The γ-tubulin ring complex (γ-TuRC) acts as a structural template for microtubule formation at centrosomes, associating with two main compartments: the pericentriolar material and the centriole lumen. The γ-TuRC has a helical shape consisting of 14 spokes, each containing a copy of γ-tubulin presented by the C-terminal gamma ring protein 2 (GRIP2) domain of one of five paralogous γ-tubulin complex proteins (GCPs). The GCP proteins interact via their N-terminal GRIP1 domains in a specific order: the γ-TuRC core harbors four pairs of GCP2/GCP3 (spoke 1–8), followed by a sequence of vertebrate-specific paralogs GCP4/GCP5/GCP4/GCP6 (spoke 9-12) and finally another pair of GCP2/GCP3 (spoke 13-14). The inside of the γ-TuRC is lined by a lumenal bridge composed of one actin molecule, as well as two α-helical modules formed by the microprotein MZT1 (mitotic-spindle organizing protein 1) and the N-terminal extensions of GCP3 and GCP6 (N-GCP3 and N-GCP6), respectively.

We subjected the purified X. laevis γ-TuRCs to cryo-EM SPA and identified a subset of particles with stoichiometric NEDD1/N-GCP3/MZT1 grapnel density. We, therefore, subjected the NEDD1/N-GCP3/MZT1 density segment to focused refinement (see “Methods”), improving local resolution for NEDD1 to 4-5 Å. The very C-terminal NEDD1 helix segments were an exception, as they were predicted straight, but are kinked in the cryo-EM reconstruction. After optimizing the model by another round of MDFF into the density obtained by focused refinement, resolved bulky hydrophobic side chains and the length of resolved alpha-helices confirmed the density segment as NEDD1. Our cryo-EM reconstruction resolves a tetramer of the NEDD1 C-terminus, comprising two consecutive helices in each protomer (NEDD1598-648 and NEDD1651-670; all residue numbers refer to X. laevis proteins). At its center, NEDD1598-648 forms a tetrameric coiled-coil that provides the binding site for four N-GCP3/MZT1 modules. The interaction between NEDD1 and the N-GCP3/MZT1 modules is characterized by complementary charged and hydrophobic patches. In addition to direct interaction with NEDD1, the N-GCP3/MZT1 modules also share an extensive interaction surface with each other, suggesting cooperative binding of N-GCP3/MZT1 modules to NEDD1. In contrast to NEDD1598-648, the NEDD1651-670 helix breaks the fourfold symmetry and forms two small dimeric coiled-coils that splay out from each other. One protomer in the upper dimer of NEDD1651-670 contacts GCP6223-240, which is part of a larger region of N-GCP6 that lines the inside of GRIP1 domains of spoke 1 and 2. The lower dimer of NEDD1651-670 appears to make little to no contact to spoke 1 and 2, but its conformation is likely stabilized by an unidentified wedge density between the upper and lower NEDD1651-670 dimers.

>MSEFRIHHDVNELISLLHVFGLEGADVYIDLLQKNRTPYVTTSVSTHSAKVKIAEFSRTPDDFLKKYEELKSKNTRNLDPLVYLLSKLIEDKETLQYLQQNAKDKAELATSSVTSVSLPIAPNTSKISMQELEELRRQLETATVAVSCSHQPVEVLRKFLRDKLNKKHTGHPVPVFPSWVYERPALTGDFMSFSNPSTDVTVSIGTLPLPSQETCLVEDLLYILIGVDGRYISVQPLVGRQSRSFSVEQNLDSSVKELVNRILPVATNYSTVTRFVEENSSFEYGQVNHALGAAMRTLGKEYMILISQLEHLQRQGLLSLQKLWFYIQPTLRTMEVLASIATSLNKGECFGGATLSLLHDRTFGYTGDSQAQELCLYLTKAASAPYFDILERWIYRGIINDPYSEFMVEEHELQKEKIQEDYNDKYWDQRYTIVQQQIPSFLQKVADKILSTGKYLNVVRECGHDVTCPDAKEITYTLKEQAYVERIEKAYNYASKVLLDFLMEEEELVAHLRSIKHYFLMDQGDFFVHFMDLTEEELKKPVDDIIPTRLEALLELALRMSTANTDPFKDDLKIELMPHDLITQLLRVLAIETHQEKALINSDPTELALSGLESFSFDYIVKWPLSLIINRKALTRYQMLFRHMFYCKHVERLLCNVWISNKTAKQFSLHSAKWFAGAFTLRQRMLNFVQNIQYYMMFEVMEPTWHILEKNLKSASNIDDVLSHHTSFLDNCLKDCMLTNPELLKIFSKLMSVCVMFTNCLQRFTQSMQVQTEMEHLTLEHGTMMGPPTQCERTEEALKKKLTSKYLEEHIDKFPSSFGFESTINNFDSNFSAHLMDLLDKLSMYSTSDCEHSMINIIYRLDFNGFYTERLKQLSSERNQKSAPLLGPAQHAVSTK[4x];>[9x]MAVPDQKSPNVLLQNLCCRILGKGEADVAQQFQYAVRVIGSNFAPTVERDEFLVTEKIKKEFVRQRREADGALFSELHRKLQSQGVLKNRWSILYLLLSLSEDPRKQPNKTSSFAALFAQALPRDAHSTPYYYARPQSLPLSYQDRNVQCAQNAASIGSSGISSIGMYALNGPTPQSIIQGQSNQTPNMGDALRQQLGSRLAWTLAAGQQPSQQSTTTKGLPNTVSRNVPRTRREGDSSGSVEITETSLVRDLLYVFQGIDGKFVKMCNSENCYKVDGKVAVSKSLKDITSKLSELGWLHNKIKKYTDQRSLDRAFGLVGQSFCAALHQELKEYYRLLSVLHSQLQVEDDQGVNLGVESSLTLRRLLVWTFDPKIRLKTLAALVDHCQGRKGGELASAVHAYTKTGDPYMRSLVQHILGLVAYPILNFLYRWIYDGELEDTYHEFFVASDPVVKTDRLWHDKYSLRKSMIPSFMTMDQSRKVLLIGKSINFLHQVCHDQTPASKAMAVGKSAESPKDAAELFTDLENAFQTKIDAAYFDTSKYLLDVLNKNYNLLEHMQAMRRYLLLGQGDFIRHLMDLLKPELVRPATTLYQHNLTGILETAVRATNAQFDNPEILKRLDVRLLEVSPGDTGWDVFSLDYHVDGPIATVFTRECMSHYLRVFNFLWRAKRMEYILTDIWKGHMCNAKLLKGMPELSGVLHQCHILASEMVHFIHQMQYYITFEVLECSWDELWNKVLKAQDLDHIIAAHDVFLDTIISRCLLDSESRALLNQLRAVFDQIIEFQNAQDALYRAALEELQQRLQFEERKKERESEGEWGVTAAEEDVENKRIQEFQESIPKMRSQLRILTHFYQGIVQQFLVLLTTSTDESLRFLSFRLDFNEHYKAREPRLRVSMGTRGRRSFHV;>MIHELLLALSGYPGSIFTWNKRTGLQVSQDIPFLHPGETSVLNRLCKLGTDYIRFTEFIEQYTGHVQQQDHHPSQQGQVGLHGIYLRAFCRGLDSILQPYRQALLDLEQEFLADPHLSISHINYSLDQFHLLFPSIMVVVEQIKSQKIHGCQILETVYKHSCGGLPPVRSALEKTLAVCHGVMYKQLSAWMLHGLLLDQYEEFFVRQGSSSGNLAAAFEEEEDDLGIGGLTGKQLRELQDLRLIEEENMLAPSLKQFSLRAEMLPSYIPVRVAEKILFVGESVQMFENQNVNMSRTGSILKNQEDTFAAELHRLKQQPLFSLVDFESVLDRIRSTVAEHLWKLMVEESDLLGQLKIIKDFYLLGRGELFQAFIDVAQNMLKTPPTAVTEHDVNVAFQLSAHKVLLDDDNLLPLLNLTIDYHGKEHKDTSQPREGPFRDMSPREAPTSGWAALGLSYKVQWPLHILFTPAVLEKYNVVFKYLLSVRRVQSELQHCWALQMQRKHLESNKTDAIKWRLQNHMAFLVDNLQYYLQVDVLESQFSQLLQQINSTRDFESIRLAHDHFLSNLLAQSFILLKPVFHCLNEILELCHSFCSLVSQNLGPLDERGAGQLDILVKGFSCQSSLLFRILSSVRNHQINPDLAQLLLRLDYNKYYTQAGGTLGSFGL[2x];> MAHWTRFERDQEGDIKKLVSLMSGIQDDQDGNFQQALQFAWSNFRFHRYLDVSSHTVLRTLEGIFEKLVVHSDLEKAESWKRLTEEFLLLPLPNTEGTKTDSHFAVLSLLLCLSDSPSNHDYTEKPRKKENDEQEPFDWGKYLREGEDIEFSPDADTPEWSEASEEEDAQEPPSREDSGIQVDRTPLEDPEKKGAPPLVSWKVGEPDARSWLEQHIVHQYWTSRAPRFSHSSHLHSNLSAIWDQHLYTTDPLYTPDDKTIVTETQVIRETLWLLSGVKKLLIFQLNDGKVNVRNDIIVTHMTQNCLRSVLEQIAAYGQVVFRLQKFIDEITGHGSEVPLPGTLPTAKKTTEAPFRTYQAFMWALYKYFISFKEELTEIEKCIINKDETVTLAIVLDKLAPRLAQLKVLHRVFSTGIAEVPPDTRNVVRASHLLNTLYKAILDYDNVGEASEQTVSLLFCLWVETVRPYLEIVDEWIVHGNLFDPAKEFIIQRNKDVPFNHRDFWYATYTLYSVSEKTENEDKMSDNASASSGSDQAPAGRQHTMVSFLKPVLKQIIMAGKSMQLLKNLKCRTALQQDSSRDSDRKSLYTLFLESVQSRLQHGNDSVPDIITEQQVNKLSLIKMQSIVAKHLELDEVHDPLLAINFVRLYLEQSDFLETFTCNEVCVDRSSESVTCQSFELTLRSCLYPHIGKQYLECCGNLMYTLKKDYRLVEYLQAMRNFFLLEAGDTMYDFYTPIFDKIREKEPWLNLSYLNVQIQEAVGQRYPDDSTRLSVSFESVDLAKKKLPVHTLDGLILSYKVPWPVDIVISSECQKIYNQVFLLLLLIKWAKYSLDVLQFNELGNASENESTKEGATVEPFPLPPLTSPSEPKGQQIHRMFLLRVKLMHFVNSLHNYLMTRILHSTGLEFQHQVEEAKDLDQLIKIHYRYLSTIHDRCLLREKVSSVKEAIMKVLNVVLMFADRWHAGLGAWKKESIVKMESDFTNCHKFLVKVLNKAVCRGSFPHLESLALSLMAGMEQS;> MDSITKLFGDLCESHMVGFPWRTALNSRKHSKNRTKQTLKKLAYDTLFVHLFQDEARKLQPNCTRLPVKNKIIMLSFNLRICGMSSEADRLEELVEYLEQSNGIQISDLHAVLELLVELSGTGPPQLLPPKRDYFKNNKYVGRNVKYQGYDYYDVQVFEADLGTTVAYQELEISTTIQRTLQIMEAAPGTGLPALSFFSQNDLSTDKFEKETRGSLFGALVHSRTNDMDIKLDMPPVPENADLSGLAIKVPQSIDQSEDEGFQSASNMTPDSQSEPSMTPDIDVWEAVLTYGPSKRRCWERIGCPPGKREEPYVTEAGREAFDKLYKLHEGGLQILSATTLQPQLVLLEETDLVKAVLNVLIGVVSSTFSYNQALQSFAVKQGVYISGTSPDNVSSLLTQVAEYGTYYTRLSHFSLLTVLDSSHSNGLVFQAFTSGLRKYLQYYRACVLSTPASLTLLTISFLFRKLGRQLRYLAELCCIGTLVTSATRGISTAFPTGVKLLSYLYKEALENSSNENYPVLLSLLKTSCEPYTRFIYDWVYSGVFRDVCGEFMIQVNEDYLGFRDKRYWTHGYVLISKEVEDCVPVFLKHVANEIYICGKTINLLKLCCPKHYICWSDIPVPRISVTFSLEELKEMEKDCAVYVARMERIARHSCISKEQKALQTEIARQELIIQARETTEKVFETFKDRKLAEKLSLDTKKRELFQKLKDQYEKEQERRLTTKQEEADDDFSYAREIRDREKRLKALEEELELKTRQELIEHYSRLSEEATRKEQRALWKLQRHKLETIRLKFFLEEQKRMQDLVANFPVDICEENLGVLPDGEISHQTDNTNDAGLGNIENEKSVPEQHALHNNNDEVYTAQNCISKSESLCVDVTLPTENVHSQTSNASVLGVPSFDSNLCTPDVDIIDFLPTLPSENQEVAVVQSLVDDALISIGSDLNTDTKDKESLCALKSDLQESSTGSEYDFKTILKPIACTQVSQGHIKIGEYSSNVQPARPRWSTHGHSSDSNIKIGNYVSDINVHQPKHSQHGHSSDSNINISDHMSDVEPRLPRLNLHGHISTGHIKVGEYASDVEPSTPRHSVHGHASQGNIKIGENVSDVKLSRPRWNIHGHVSDANIKIGENTSEIAPLRPRWNIHGHASQSHIKIGELVSDIEPSQPRRTPFGHPSQSSIPIGDQPVEKYAQKSESEVHSSNSTIQHLLYSNIPDKNKDTGGTLTDSPVPVPDQGNSNDDTEKRSSTLEQRVQAADSVCDGEASPNTAQSLPCMSDTLDFGTNGEENVGNDDHTWEKQQEYLKGLAEKYCLEKYQDSYELMSHPPVLHLYSNVMPNRFSFPTDSDIKSATDETTVQLIELLSLPVLMKYSVTAPMVSHVYLVNKAIVDYYFVELKMERHFEAMRHFLLMEDGEFAQSLSDMLFEKLGSGQTPSELLNPLVLNSILNKALQYSLHGDSSLASNLTFALKYLPEVFTPTAPDALSCLELKYKVDWPLNIVITDTCMNKYSRIFSFLLQLKHMVWTLRDVWFHLKRTALVNQASNSVQYRQLQLYRHEMQHFVKVIQGYIANQILHVTWCEFRNKLSAVSNLEEIYKTHADYLNKALFRGLLTEKAAPLMNIIHSIFSLILKFRLQLISQSWICDTGKQMAVHPNFGLMQQSYNTFKYYSDFLFEVVSKLVNRGYQPHLEDFLLRINFNSYYKQS;>[4x]MESRGGGGRVRLPGTTMQDNIRFVSAGDDVKIWDYSSMTTVEQFNPHSASHPVSSLCWSSNNHFLVTASGSGDKIVVSSCKSKPVPLLELAEGKKQTCVNLNSSSQYVVSGGLDNTVNIWDLKSKRLHRSLKDHKDEVTCVTFNANDCYVASGSMSGEIILHNVTTNLSSTPFGHGSSQPIRHLKYSYVKKSLLGTVSDSGSVTLWDANSQNPYHVFESAHKAPASGICFSPVNDLLLVTVGLDKRIICYDVSSKILLQTVVAESPLTAVDFMPDGATLAVGSSRGKIYLYDLRMLSSPVKTVSAHKTSVQCIQFQHSNIYKSSKGPSSKSSILSTAVNKKPSTKTAAGGTQSANITKDLPPSAISSLPQPVMPVDSKVLRVNDDKSGFPRSTSLDIIPSKETDFAKTSDYKSIDSFGRSSLGDIFSPVRDDASHFRGAEDLSCKGNDLDYLPQFSTIPSSRRNPVGANTQGIHGSPLHLIIESPIKEEDESQDSELKTRKPQLLKQDFRESSSKPASVDQNNLNNSPINSVTRTPEAIEKTGHQILSQLKSDVPAHGTKIASPKVAATMSTQLASSLSEKIADTLASDRTGAPLTAIQINFIKNMIEETLDDFREACHRDIVNLQVEMIKQFHIQSSEIQMLLERYSLNESLVSEIEKLREENKRLRANF;>MANASGNMSAVRETMDVLLEISRLLNTGLDMETLSICVRLCEQGINPEALSSVIKELRRASDTLKASESTAS[6x]> MACNK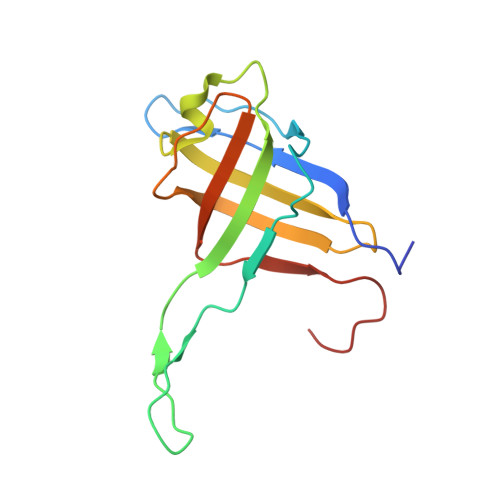QNGVKNILITFTHCDTGEVIGPISHEQPDDTLPTYKTCAWTNTALTNGAVMRSASNATMTLPVVRDPRVPLAWYQGCAQIDAQVEKFDGTVMTLTEGAVTEPEESDGRAVTMTIIAAEIDELLPPGSLAAA>[2x]MARKWLNLFAGAALSFAVAGNALADEGKITVFAAASLTNAMQDIATQFKKEKG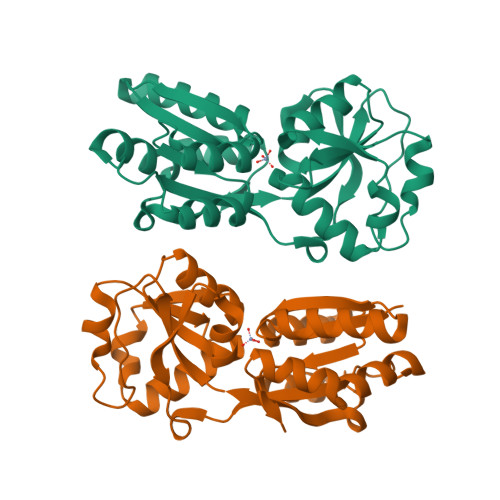VDVVSSFASSSTLARQIEAGAPADLFISADQKWMDYAVDKKAIDTATRQTLLGNSLVVVAPKASVQKDFTIDSKTNWTSLLNGGRLAVGDPEHVPAGIYAKEALQKLGAWDTLSPKLAPAEDVRGALALVERNEAPLGIVYGSDAVASKGVKVVATFPEDSHKKVEYPVAVVEGHNNATVKAFYDYLKGPQAAEIFKRYGFTIK>[2x]MSLRSDLINALYDENQKYDVCGIISAEGKIYPLGSDTKVLSTIFELFSRPIINKIAEKHGYIV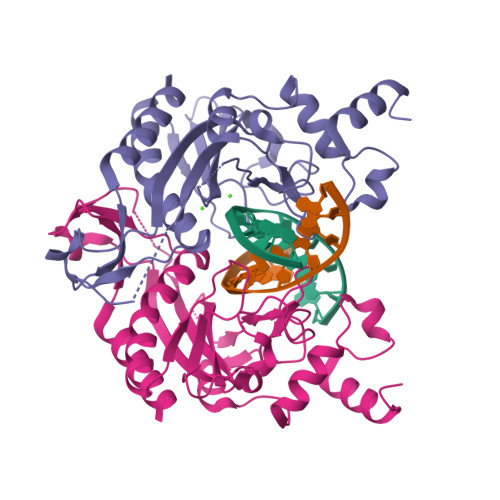EEPKQQNHYPDFTLYKPSEPNKKIAIDIKTTYTNKENEKIKFTLGGYTSFIRNNTKNIVYPFDQYIAHWIIGYVYTRVATRKSSLKTYNINELNEIPKPYKGVKVFLQDKWVIAGDLAGSGNTTNIGSIHAHYKDFVEGKGIFDSEDEFLDYWRNYERTSQLRNDKYNNISEYRNWIYRGRK>[4x]MAPTSSIEIVLDKTTASVGEIVTASINIKNITNFSGCQLNMK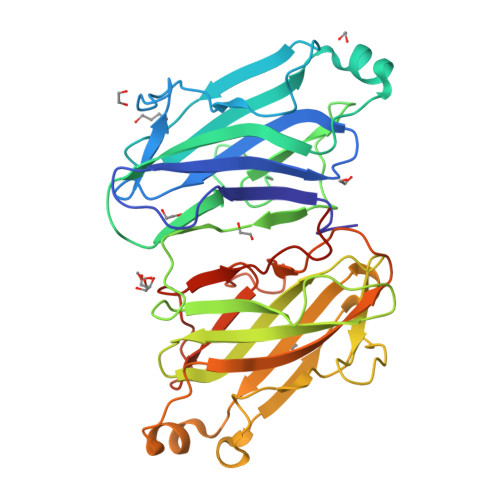YDPAVLQPVTSSGVAYTKSTMPGAGTILNSDFNLRQVADNDLEKGILNFSKAYVSLDDYRTAAAPEQTGTVAVVKFKVLKEETSSISFEDTTSVPNAIDGTVLFDWNGDRIQSGYSVIQPAVINLDMTKASYITMGYDKNAAEVGEIIKATVKINKITNFSGYQVNIKYDPTVLQAVNPKTGVAYTNSSLPTSGELLVSEDYGPIVQGVHKISEGILNLSRSYTALEVYRASESPEETGTLAVVGFKVLQKKATTVVFEDSETMPNGITGTTLFNWYGNRIQSGYFVIQPGEINSAPIATLEHHHHHH>[3x]AQVINTFDGVADYLQTYHKLPD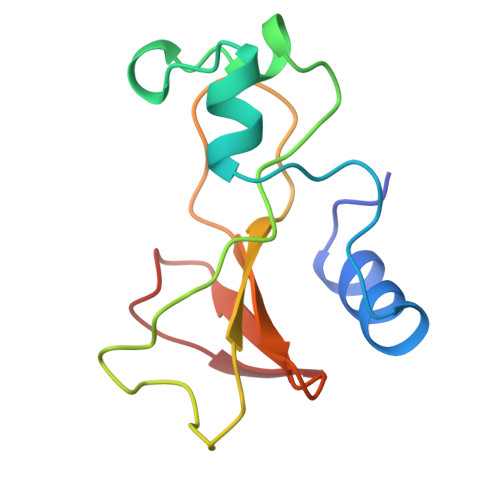NYITKSEAQALGWVASKGNLADVAPGKSIGGDIFSNREGKLPGKSGRTWREADANYTSGFRNSDRILYSSDWLIYKTTDHYQTFTKIR>[2x]GAMGSEEKLREVSSQDPVTGLYNRSHFLDLMDAAVQQAVTARKPSTLAYIHLNGYPSLQADHGLSGIDLLLGQLAGLMREQFGEEADLARFGDSIFAALFKGKTPEQAQAALQRLLKKVENHLFELNGRSAQATLSIGVAGLDEKTAKAQDVMNRAHR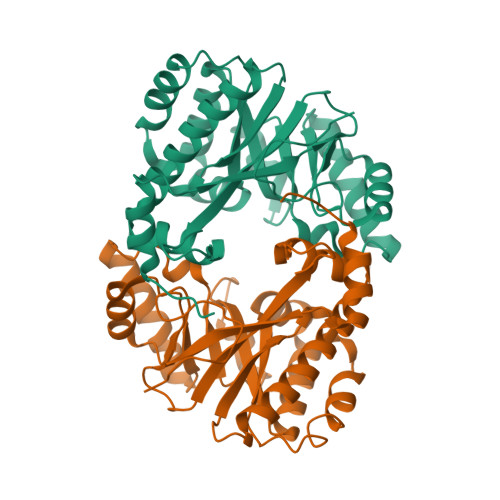CADDAARKGGSQIKQYNPAEELAAAAQRGDVIAILQQALETNSFRLLFQPVISLRGDSHENYEVLLRLLNPQGQEVPPAEFLHAAKEAGLAEKIDRWVILNSIKLLAEHRAKGHQTKLFVHLSSASLQDPGLLPWLGVALKAARLPPESLVFQISEADATSYLKQAKQLTQGLATLHCQAAISQFGCSLNPFNALKHLTVQFIKIDGSFVQDLNQVENQEILKGLIAELHEQQKLSIVPFVESASVLATLWQAGATYIQGYYLQGPSQAMDYDFSSGDE> NLYFQGHMDNVDELRKIENKSSFVSADNMPEYVKGAFISMQDERFYNHHGFDLKGTTRALFSTISDRDVQGGSTITQQVVKNYFYDNDRSFTRKVKELFVAHRVEKQYNKNEILSFYLNNIYFGDNQYTLEGAANHYFGTTVNKNSTTMSHITVLQSA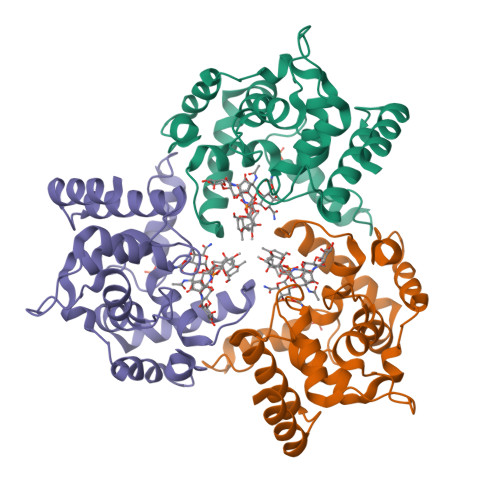ILASKVNAPSVYNINNMSENFTQRVSTNLEKMKQQNYINETQYQQAMSQLN> MKTIGLLGGMSWESTIPYYRLINEGIKQRLGGLHSAQVLLHSVDFHEIEECQRRGEWDKTGDILAEAALGLQRAGAEGIVLCTNTMHKVADAIESRCTLPFLHIADATGRAITGAGMTRVALLGTRYTMEQDFYRGRLTEQFSINCLIPEADERAKINQIIFEELCLGQFTE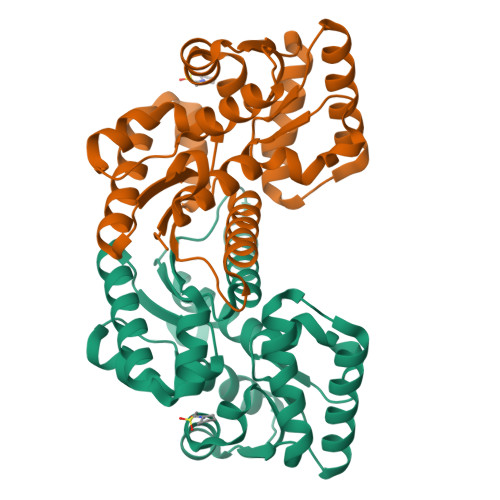ASRAYYAQVIARLAEQGAQGVIFGCTEIGLLVPEERSVLPVFDTAAIHAEDAVAFMLSLEHHH>[2x]MGSSHHHHHHSSGLVPRGSHMSPSPVPGSQNVPAPAVKKISQYACQRRTTLNNYNQLFTDALDILAENDELRENEGSCLAFMRASSVLKSLPFPITSMKDTEGIPCLGDKVKSIIEGII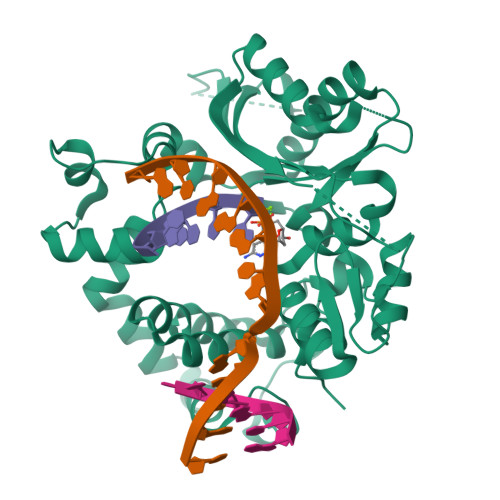EDGESSEAKAVLNDERYKSFKLFTSVFGVGLKTAEKWFRMGFRTLSKIQSDKSLRFTQMQKAGFLYYEDLVSCVNRPEAEAVSMLVKEAVVTFLPDALVTMTGGFRRGKMTGHDVDFLITSPEATEDEEQQLLHKVTDFWKQQGLLLYHQYHRSHLADSAHNLRQRSSTMDVFERSFCILKLDHGRVHSEKSGQQEGKGWKAIRVDLVMCPYDRRAFALLGWTGSRQFERDLRRYATHERKMMLDNHALYDRTKRVFLEAESEEEIFAHLGLDYIEPWERNA> QPDPKLDELNKVSDYKSNKGTMGNVMNLYMSPPVEGRGVINSRQFLSHDLIFPIEYKSYNEVKTEL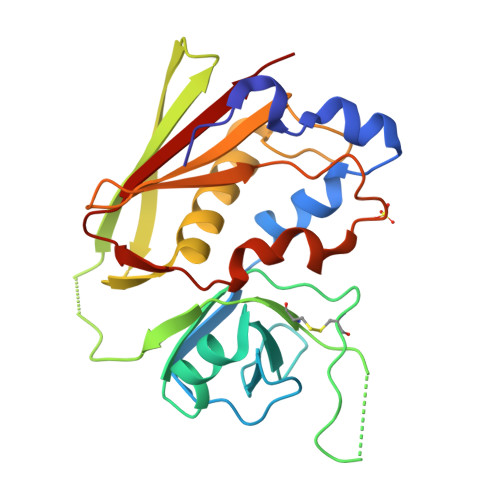ENTELANNYKGKKVDIFGVPYFYTCIIPKSEPDINQNFGGCCMYGGLTFNSSENERDKLITVQVTIDNRQSLGFTITTNKNMVTIQELDYKARHWLTKEKKLYEFDGSAFESGYIKFTEKNNTSFWFDLFPKKELVPFVPYKFLNIYGDNKVVDSKSIKMEVFLNTH>[2x]MATPASAPDTRALVADFVGYKLRQKGYVSGAGPGEGPAADPLGQALRAIGDEFETRFRRTFSDLAAQLHVTPGSAQQRFTQVSDELFQGGPNWGRLVAFFVFGAALCAESVNKEME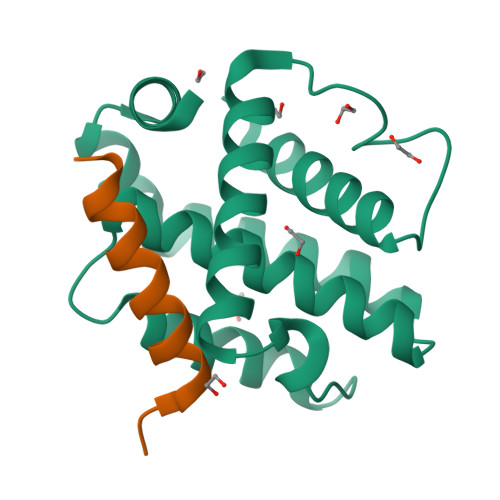PLVGQVQEWMVEYLETRLADWIHSSGGWAEFTALYGDGALEEARRLR;>[2x]AADPLGQALRAIGDEFETRFR>[2x]MNIYRYEENPLITPLDVKPIHEGFEVIGAFNGGVAEYNGEVLLLLRVAEKPVSEDPEIVLAPVYNAKNKELELQSFRLDDENYDFEDPRMIRSKAKLEGFSYLTSLSYIRIARSKDGHHFTLDEKPFLY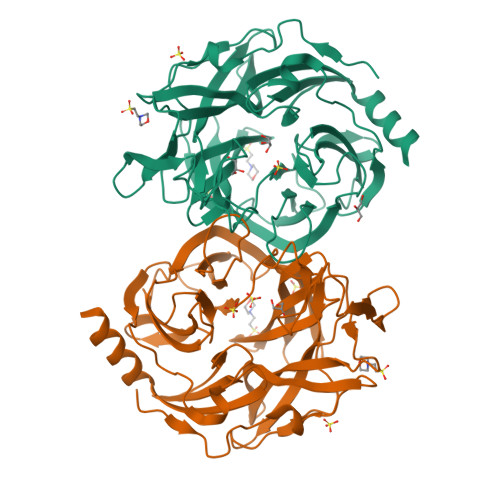PFNEYQTFGIEDARVTQIGDTYHVNFSAVSEFGVADALVTTKDFENLEYQGNIFAPENKDVLIFPEKINGKYYALHRPSLKSIGNLDIWIASSPDLRSFGDHRHLLGIRPGEYDSGRVGGGCVPIKTEEGWLILYHGATEENRYVMGAALLDLNDPTIVLKRTKTPILEPVADYEKNGFFGDVVFACGAIQEGDTLHMYYGVADTSMAGCDMKISEILHQLEVEAKLEHHHHHH> SLTFYPAWLTVSEGANATFTCSLSNWSEDLMLNWNRLSPSNQTEKQAAFSNGLSQPVQDARFQIIQLPNRHDFHMNILDTRRNDSGIYLCGAISLHPKLKIEESPGAELVVTERILE;> LFTVTAPKEVYTVDVGSSVSLECDFDRRECTELEGIRASLQKVENDTSLQSERATLLEEQLPLGKALFHIPSVQVRDSGQYRCLVICGAAWDYKYLTV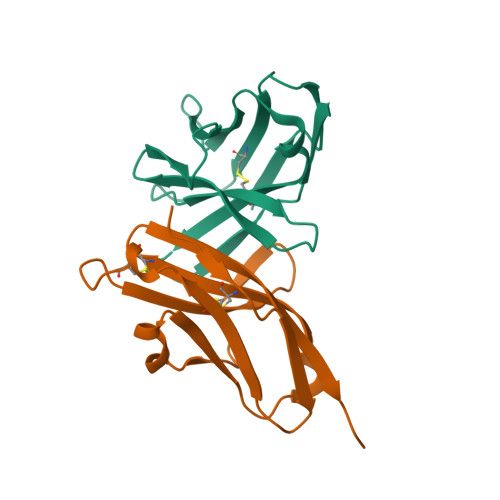KVKASY> MAKTLKDLQGWEIITTDEQGNIIDGGQKRLRRRGNKTEHYLKRSSDGIKLGRGDSVVMHNEAAGTYSVYMIQELRLNTLNNVVELWALTYLRWFEVNPLAHYRQFNPDANILNRPLNYYNKLFSETANKNELYLTAELAELQLFNFIRVANVMDGSKWEVLKGNVDPERDFTVRYICEPTGEKFVDINIEDVKAYIKKVEPREAQEYLKDLTLPSKKKE;> EKKFSTEEEYVSPRFLVADGFLIDLAEEKPINPKDPRLLTLLKDHQRAMIDQMNLVKWNDFKKYQDPIPLKAKTLFKFCKQIKKKFLRGADFKLHTLPTEANLKYEPERMTVLCSC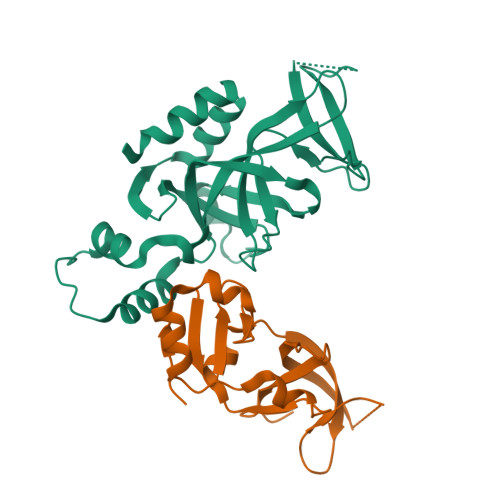VPILLDDQTVQYLYDDSLEHHHHH> MGSSHHHHHHHHLEVLFQGPHMASLQRKGLQARILTSEEEEKLKRDQTLVSDFKQQKLEQEAQKNWDLFYKRNSTNFFKDRHWTTREFEELRSCREFEDQKLTMLEAGCGVGNCLFPLLEED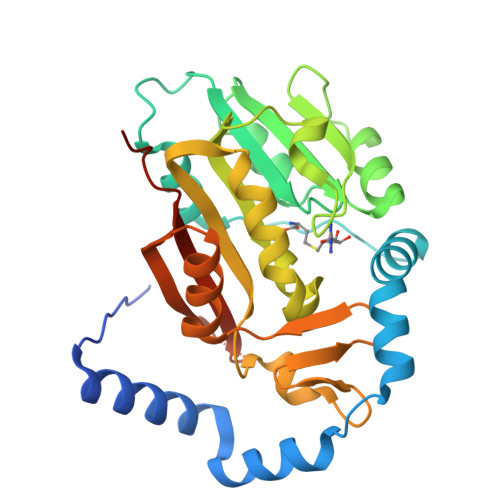PNIFAYACDFSPRAIEYVKQNPLYDTERCKVFQCDLTKDDLLDHVPPESVDVVMLIFVLSAVHPDKMHLVLQNIYKVLKPGKSVLFRDYGLYDHAMLRFKASSKLGENFYVRQDGTRSYFFTDDFLAQLFMDTGYEEVVNEYVFRETVNKKEGLCVPRVFLQSKFLKPPKNPSPVVLGLDPKS>MIVVKVGGAEGINYEAVAKDAASLWKEGVKLLLVHGGSAETNKVAEALGHPPRFLTHPGGQVSRLTDRKTLEIFEMVYCGLVNKRLVELLQKEGANAIGLSGLDGRLFVGRRKTAVKYVEN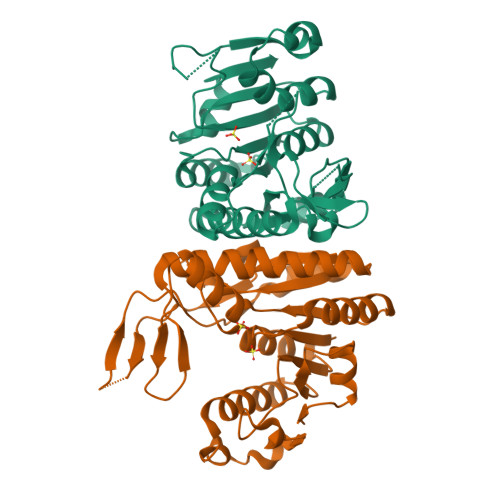GKVKVHRGDYTGTVEEVNKALLDLLLQAGYLPVLTPPALSYENEAINTDGDQIAALLATLYGAEALVYLSNVPGLLARYPDEASLVREIPVERIEDPEYLALAQGRMKRKVMGAVEAVKGGVKRVVFADGRVENPIRRALSGEGTVVR[2x]> MDTTRFIRNFILFKDALQKQNFNNKDLNTTSMQAALQSEQLALSEESQYLQSEQVRAKMQIDFLGMQANLQN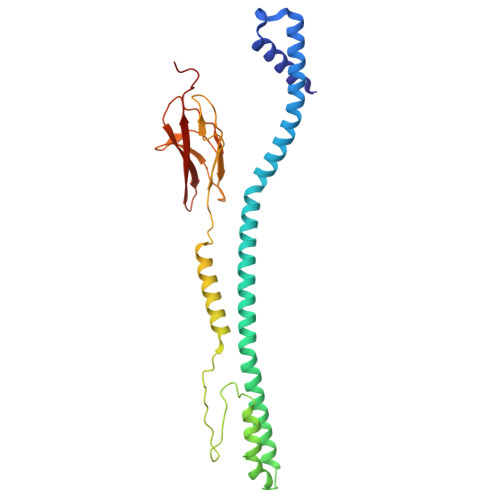AKAETLNKLIQCQAMLKSLKDNAMINRANALVSLLQVQANAANGITTSNFEAAFKIIAQIGSEYNQITLNNGNVSVQEKEQTNELKTILNSLSKELEKLNQQSEVNSIQIFSDKLEVLKDAPARLWGFSTLSNAKEGFYNEANEQIASGSVCLFRSDKVRKHTITFKAINTKTSLSKNITISVIANKLKERMS>[2x]GAPIANELRCQCLQTMAGIHLKNIQSLCVLPSGPHCTQTEVIATLKNGREACLDP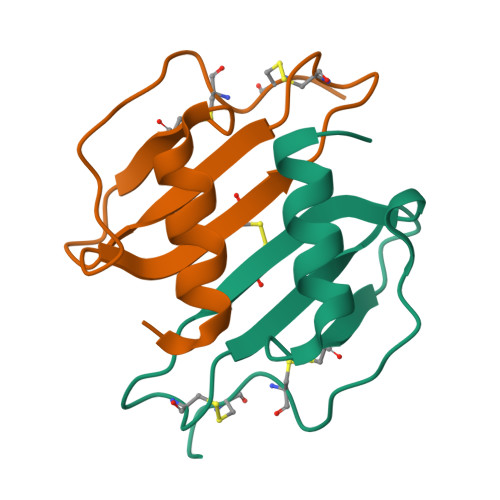EAPLVQKIVQKMLKGVPK> MIDVIMTGELLKTVTRAIVALVSEARIHFLEKGLHSRAVDPANVAMVIVDIPKDSFEVYNIDEEKTIGVDMDRIFDISKSISTKDLVELIVEDESTLKVKFGSVEYKVALIDPSAIRKEPRIPELELPAKIVMDAGEFKKAIAAADKISDQVIFRSDKEGFRIEAKGDVDSIVFHMTETE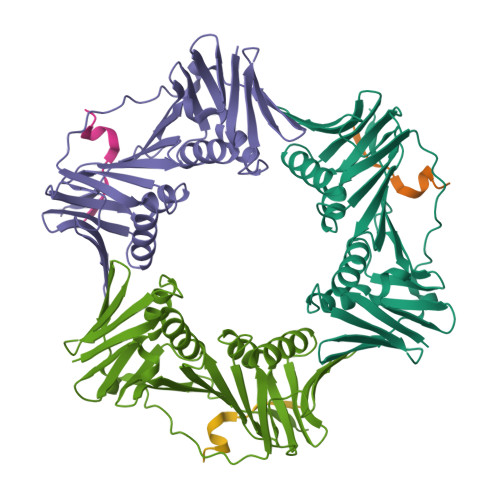LIEFNGGEARSMFSVDYLKEFCKVAGSGDLLTIHLGTNYPVRLVFELVGGRAKVEYILAPRIESE;> KTTQSTLDSFFK> MELKHSISDYTEAEFLQLVTTICNADTSSEEELAKLVTHFEEMTEHPSGSDLIYYPKEGDDDSPSGIVNTVKQWRAANGKSG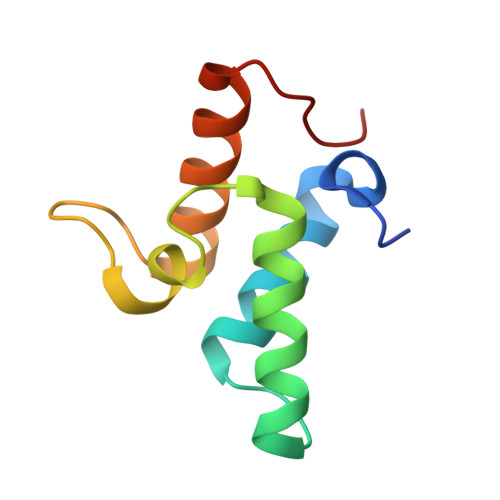FKQG>[3x]MNEQIPHDKSLDNSLTLLKEGYLFIKNRTERYNSDLFQARLLGKNFICMTGAEAAKVFYDTDRFQRQNALPKRVQKSLFGVNAIQGMDGSAHIHRKMLFLSLMTPPHQKRLAELMTEEWKAAVTRWEKADEVVLFEEAKEILCRVACYWAGVP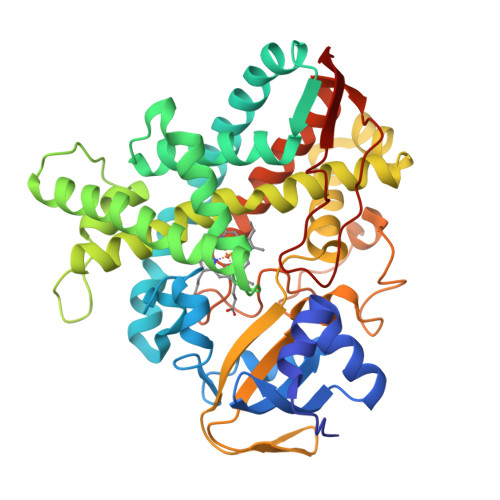LKETEVKERADDFIDMVDAFGAVGPRHWKGRRARPRAEEWIEVMIEDARAGLLKTTSGTALHEMAFHTQEDGSQLDSRMAAIELINVLRPIVAISYFLVFSALALHEHPKYKEWLRSGNSREREMFVQEVRRYYPFGPFLGALVKKDFVWNNCEFKKGTSVLLDLYGTNHDPRLWDHPDEFRPERFAEREENLFDMIPQGGGHAEKGHRCPGEGITIEVMKASLDFLVHQIEYDVPEQSLHYSLARMPSLPESGFVMSGIRRKS> MSAPTPLAEASQIPTIPALSPLTAKQSKGNFFSSNPISSFVVDTYKQLHSHRQSLELVNPGTVENLNKEVSRDVFLSQYFFTGLRADLNKAFSMNPAFQTSHTFSIGSQALPKYAFSALFANDNLFAQGNIDNDLSVSGRLNYGWDKKNISKVNLQISDGQPTMCQLEQDYQASDFSVNVKTLNPSFSEKGEFTGVAVASFLQSVTPQLALGLETLYSRTDGSAPGDAGVSYLTRYVSKKQDWIFSGQLQANGALIASLWRKVAQNVEAGIETTLQAGMVPITDPLMGTPIGIQPTVEGSTTIGAKYEYRQSVYRGTLDSNGKVACFLERKVLPTLSVLFCGEIDHFKNDTKIGCGLQFETAGNQELLMLQQGLDAD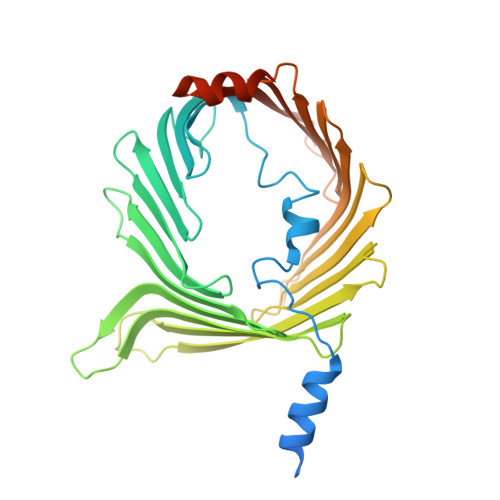GNPLQALPQLGGWSHPQFEK2-[3-[(1~{R})-1-[(2~{S})-1-[(2~{S})-2-(5-chloranylthiophen-2-yl)pent-4-enoyl]piperidin-2-yl]carbonyloxy-3-(3,4-dimethoxyphenyl)propyl]phenoxy]ethanoic acid 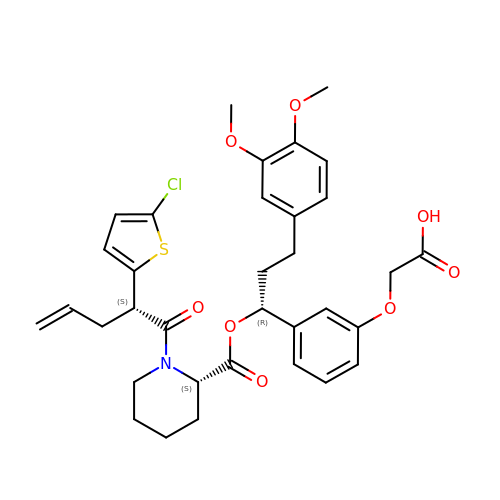| C34 H38 Cl N O8 S | NEIWCSGIZZQIHO-KWXIBIRDSA-N>MMKPEDVIKEQCARAKVVAELWHGFTGGAPKAALENLVVEFNKAQQGRCVRPVPQGGYRDLSTKIKAAFAAGKVPTMAQAFENNIALYLEAKALLPIESLGVKLQGVNLTFLNAVRFGGVVYGVPFNKSIQVLYYNKDLLKKHGVPVPATLEEFVAAAKKLSRAEGGPVYWFQPDASTFAYFFFNLGGSYLKDGKLVLNSK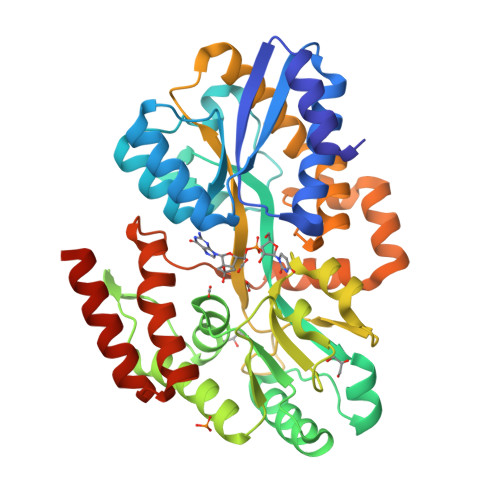EAVEALTLLQNGVKEGWAKPITSGYINQNLGSGPYAFSVDTSAGYTAYLRAAKFDLGVATLPGRTKGQPGYGLVQGTNLVVFRQASKEEQAVAKDFLEFVLSPRAQAVFATATGYVPVTEGALKDPVYQAYAAENPDYATIVRQSRYAKFEPALAEWEQIRFDILGQAIKEAILNKADPKAALDRAQKLAEDLLSSRTRHHHHHH[2x]>[2x]HHHPCCSNPCQNRGECMSTGFDQYKCDCTRTGFYGENCTTPEFLTRIKLLLKPTPNTVHYILTHFKGVWNIVNNIPFLRSLIMKYVLTSRSYLIDSPPTYNVHYGYKSWEAFSNLSYYTRALPPVADDCPTPMGVKGNKELPDSKEVLEKVLLRREFIPDPQGSNMMFAFFAQHFTHQFFKTDHKRGPGFTRGLGHGVDLNHIYGETLDRQHKLR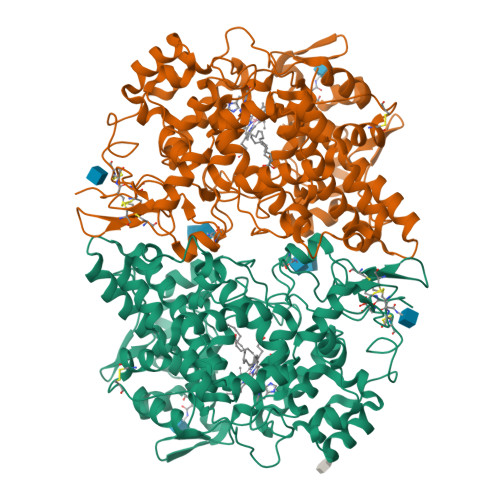LFKDGKLKYQVIGGEVYPPTVKDTQVEMIYPPHIPENLQFAVGQEVFGLVPGLMMYATIWLREHNRVCDILKQEHPEWGDEQLFQTSRLILIGETIKIVIEDYIQHLSGYHFKLKFDPELLFNQQFQYQNRIASEFNTLYHWHPLLPDTFNIEDQEYSFKQFLYNNSILLEHGLTQFVESFTRQIAGRVAGGRNVPIAVQAVAKASIDQSREMKYQSLNEYRKRFSLKPYTSFEELTGEKEMAAELKALYSDIDVMELYPALLVEKPRPDAIFGETMVELGAPFSLKGLMGNPICSPQYWKPSTFGGEVGFKIINTASIQSLICNNVKGCPFTSFNV> MSFSDQNLIWIDLEMTGLDPEMHKIIEMATIVTDSELNILAEGPVIAIHQPESELAKMDEWCTTTHTASGLVARVRQSQVSEEEAIDQTLAFLKQWVPEGKSPICGNSIGQDRRFLYKHMPRLEAYFHYRYIDVSTIKELTRRWQPEV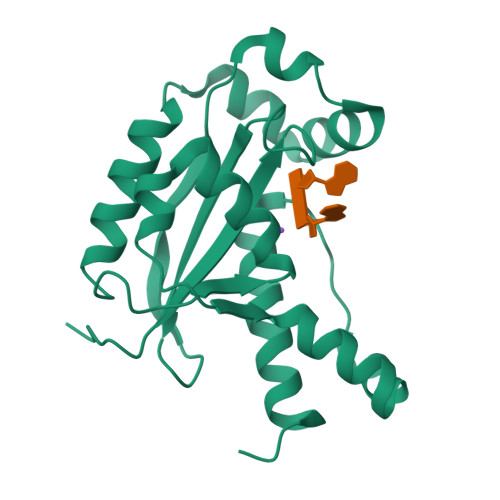LKEFSKTGSHLALDDIRESIAELQFYRKAVFKI>[2x]ATFEIVNRCSYTVWAAASKGDAALDAGGRQLNSGESWTINVEPGTNGGKIWARTDCYFDDSGSGICKTGDCGGLLRCKRFGRPPTTLAEFSLNQ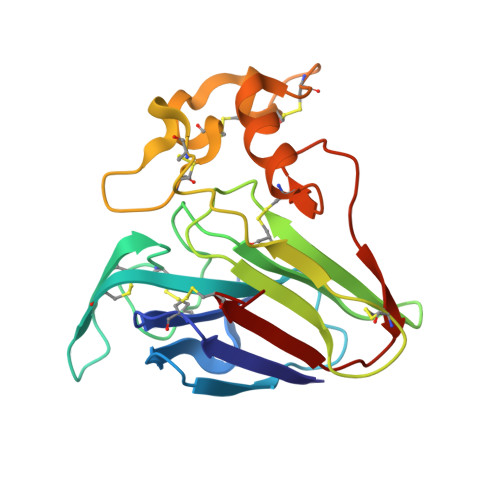YGKDYIDISNIKGFNVPMNFSPTTRGCRGVRCAADIVGQCPAKLKAPGGGCNDACTVFQTSEYCCTTGKCGPTEYSRFFKRLCPDAFSYVLDKPTTVTCPGSSNYRVTFCPTA AmicoTA is a transaminase of PLP fold type IV, which is active toward D-amino acids and α-keto acids. Transaminases (TAs, aminotransferases, EC 2.6.1) are well-established in large-scale chemistry. These are pyridoxal-5′-phosphate (PLP)-dependent enzymes that catalyze the stereoselective transfer of an amino group from an amino donor (amine or amino acid) to a keto compound (ketone, keto acid, or aldehyde) to form new amino and keto products. The catalytic unit of TAs is a homodimer, with two active sites formed by the amino acid residues of both subunits. Each subunit of the dimer consisted of two α/β domains: a small domain (residues 1–114) and a large domain (residues 127–275), connected by the interdomain loop (residues 115–126).

To shed light on the substrate binding mode in AmicoTA, the structure with D-glutamate was obtained at 1.9Å resolution. In the complex D-glutamate is covalently bound with PLP via Schiff linkage. Considering that the dihedral angle C3-C4-C4′-N4′ is 60° and 40° in subunits A and B, respectively, the adduct between D-glutamate and PLP is a ketimine rather than an aldimine. The occupancy of the adduct was found to be 0.7, the rest of the cofactor was in PMP form. The pyridine ring was tilted 15° from its position in the holoenzyme around the N1-C6 bond, and the released side chain of the catalytic lysine moved toward Y146, forming a hydrogen bond between its εNH2 group and OH group of Y146. The α-carboxylate group of D-glutamate formed a salt bridge with the guanidine group of R27* and a hydrogen bond with the hydroxyl group of T34. Backbone nitrogen atoms of V236 and K237 as well as the Nε atom of the latter coordinated the γ-carboxylate group of D-glutamate. Neither K99* with H101* (analogs of the “carboxylate trap” in bsDAAT) nor R116 was found to participate in the substrate binding. To summarize, no canonical “carboxylate trap” was formed when D-glutamate entered the active site.

>GHMNLCYIDGKFLPLEEAKLPVTDLIIQRGVGVFETISTHSRRPLMLTPHLKRLEGSATASSIVMPATLDEMARIIREGIKKMGCETMVRPYITGGDSFGKDHLFSSSRYFVIFEEIRKPDPILYEKGVALHPINAERYLPSTKSINYMLSFTGQRDSKGAYEILYCPEGEIVEGSHSTFFLIKNGHLITAPTSRALSGTTRQIVLELARRGNIQVEERCPLLTELPEAEEAFITGTVKELLPVVRIGDQIIGNGVPGKLTKHLHQVYLSSIVEWLE[2x]>NIFEXQVDAQPLRPCELQRERAFLKREDYVPQCAEDGSFQTVQCGKDGASCWCVDADGREVPGSRQPGRPAACLSFCQLQKQQILLSSYINSTATSYLPQCQDSGDYSPVQCDLRRRQCWCVDAEGMEVYGTRQQGRPARCPRSCEIRNRRLLHGVGDRSPPQCSPDGAFRPVQCKFVNTTDMMIFDLVHSYSRFPDAFVTFSSFRSRFPEVSGYCYCADSQGRELAETGLELLLDEIYDTIFAGLDLASTFAETTLYRILQRRFLAVQLVISGRFRCPTKCEVERFAATSFRHPYVPSCHPDGEYQAAQCQQGGPCWCVDSRGQEIPGTRQRGEPPSCAEDQSCPSERRRAFSRLRFGPSGYFSRRSLLLAPEEGPVSQRFARFTASCPPSIKELFLDSGIFQPMLQGRDTRFVAPESLLKEAIRGLFPSRELARLALQFTTNAKRLQQNLFGGRFLVNVGQFNLSGALGTRGTFNFSHFFQQLGLPGFQDGRALADLAKPLSVGLNSNPASEAPKASKIDVALRKPVVGSFGFEVNLQENQNALQFLSSFLELPEFLLFLQHAISVPEDIARDLGDVMEMVFSSQGCGQAPGSLFVPACTAEGSYEEVQCFAGDCWCVDAQGRELAGSRVRGGRPRCPTECEKQRARMQSLLGSQPAGSSLFVPACTSKGNFLPVQCFNSECYCVDTEGQPIPGTRSALGEPKKCPSPCQLQAERAFLGTVRTLVSNPSTLPALSSIYIPQCSASGQWSPVQCDGPPEQAFEWYERWEAQNSAGQALTPAELLMKIMSYREAASRNFRLFIQNLYEAGQQGIFPGLARYSSFQDVPVSVLEGNQTQPGGNVFLEPYLFWQILNGQLDRYPGPYSDFSAPLAHFDLRSCWCVDEAGQKLEGTRNEPNKVPACPGSCEEVKLRVLQFIREAEEIVTYSNSSRFPLGESFLAAKGIRLTDEELAFPPLSPSRETFLEKFLSGSDYAIRLAAQSTFDFYQRRLVTLAESPRAPSPVWSSAYLPQCDAFGGWEPVQCHAATGHCWCVDGKGEYVPTSLTARSRQIPQCPTSCERLRASGLLSSWKQAGVQAEPSPKDLFIPTCLETGEFARLQASEAGTWCVDPASGEGVPPGTNSSAQCPSLCEVLQSGVPSRRTSPGYSPACRAEDGGFSPVQCDPAQGSCWCVLGSGEEVPGTRVAGSQPACESPQCPLPFSVADVAGGAILCERASGLGAAAGQRCQLRCSQGYRSAFPPEPLLCSVQRRRWESRPPQPRACQRPQFWQTLQTQAQFQLLLPLGKVCSADYSGLLLAFQVFLLDELTARGFCQIQVKTAGTPVSIPVCDDSSVKVECLSRERLGVNITWKLQLVDAPPASLPDLQDVEEALAGKYLAGRFADLIQSGTFQLHLDSKTFSADTSIRFLQGDRFGISPRTQFGCLEGFGRVVAASDASQDALGCVKCPEGSYFQDEQCIPCPAGFYQEQAGSLACVPCPEGRTTVYAGAFSQTHCVTDCQKNEVGLQCDQDGQYRASQRDRTSGKAFCVDGEGRRLPWTEAEAPLVDAQCLVMRKFEKLPESKVIFSADVAVMVRSEVPGSESSLMQCLADCALDEACGFLTVSTAGSEVSCDFYAWASDSIACTTSGRSEDALGTSQATSFGSLQCQVKVRSREGDPLAVYLKKGQEFTITGQKRFEQTGFQSALSGMYSPVTFSASGASLAEVHLFCLLACDHDSCCDGFILVQVQGGPLLCGLLSSPDVLLCHVRDWRDPAEAQANASCPGVTYDQDSRQVTLRLGGQEIRGLTPLEGTQDTLTSFQQVYLWKDSDMGSRSESMGCRRDTEPRPASPSETDLTTGLFSPVDLIQVIVDGNVSLPSQQHWLFKHLFSLQQANLWCLSRCAGEPSFCQLAEVTDSEPLYFTCTLYPEAQVCDDILESSPKGCRLILPRRPSALYRKKVVLQDRVKNFYNRLPFQKLTGISIRNKVPMSDKSISSGFFECERLCDMDPCCTGFGFLNVSQLKGGEVTCLTLNSLGLQTCSEEYGGVWRILDCGSPDTEVRTYPFGWYQKPVSPSDAPSFCPSVALPALTENVALDSWQSLALSSVIVDPSIRNFDVAHISTAAVGNFSAARDRCLWECSRHQDCLVTTLQTQPGAVRCMFYADTQSCTHSLQAQNCRLLLHEEATYIYRKPNIPLPGFGTSSPSVPIATHGQLLGRSQAIQVGTSWKPVDQFLGVPYAAPPLGEKRFRAPEHLNWTGSWEATKPRARCWQPGIRTPTPPGVSEDCLYLNVFVPQNMPPNASVLVFFHNAAEGKGSGDRPAVDGSFLAAVGNLIVVTASYRTGIFGFLSSGSSELSGNWGLLDQVVALTWVQTHIQAFGGDPRRVTLAADRGGADIASIHLVTTRAANSRLFRRAVLMGGSALSPAAVIRPERARQQAAALAKEVGCPSSSVQEMVSCLRQEPARILNDAQTKLLAVSGPFHYWGPVVDGQYLRETPARVLQRAPRVKVDLLIGSSQDDGLINRAKAVKQFEESQGRTSSKTAFYQALQNSLGGEAADAGVQAAATWYYSLEHDSDDXASFSRALEQATRDYFIICPVIDMASHWARTVRGNVFMYHAPESYSHSSLELLTDVLYAFGLPFYPAYEGQFTLEEKSLSLKIMQYFSNFIRSGNPNYPHEFSRRAPEFAAPWPDFVPRDGAESYKELSVLLPNRQGLKKADCSFWSKYIQSLKASADETKDGPSADSEEEDQPAGSGLTEDLLGLPELASKTYSK[2x]

Thyroglobulin (Tg) is a 660 kDa (2 × 330 kDa) homodimeric protein which is the most highly expressed protein in the thyroid gland. The protein is secreted by thyrocytes into the thyroid follicle lumen where, upon iodination by thyroid peroxidase, Tg functions as a scaffold protein for thyroid hormonogenesis and as a storage protein for both thyroid hormones and iodide. An oxidative coupling reaction in which a diiodotyrosine (DIT) acceptor receives (via a covalent quinol-ether linkage) the iodophenolic ring of a neighboring DIT donor results in the formation of thyroxine at an acceptor site and dehydroalanine at the corresponding donor site. Tg is a homodimeric protein packed with multiple Tg type 1 (Tg1) repeating structural motifs.

Here, a three-dimensional cryoEM reconstruction of bovine thyroglobulin at an overall resolution of 2.6 Å is presented. In this report, we present a high-resolution structure of purified Tg (iodinated in vivo with normal iodide content) from the bovine thyroid gland. We have been able to definitively identify three (of 70) tyrosine side chains per Tg monomer that are modified either to diiodotyrosine or thyroxine (Tyr24 and Tyr2575, indicative of acceptor sites). In addition, we observe four tyrosines with no discernible side chain despite well defined main-chain density, which we have tentatively assigned as dehydroalanines (Tyr89, Tyr149, Tyr1395 and Tyr2542); these are the only identifiable candidates as donors in thyroid hormone formation. Nevertheless, two acceptor–donor pairs were clearly identified in the structure, involving Tyr24 (acceptor)–Tyr149 (donor) and Tyr2542 (donor)–Tyr2575 (acceptor). Our high-resolution cryoEM map and model provide clear structural evidence for Tyr24–Tyr149 and Tyr2575–Tyr2542 functioning as acceptor–donor pairs. Both thyroxine acceptor sites at Tyr24 and Tyr2575 exhibited extra densities in the cryoEM map, revealing two phenolic rings coupled together, forming T4 at the site of the acceptor tyrosine. In contrast, Tyr149 exhibited no side-chain density in the cryoEM map, likely indicating the conversion of Tyr149 to dehydro­alanine. The distance between the Tyr24–Tyr149 acceptor–donor pair is 27.4 Å (Cα–Cα) in our structure in which thyroxine has already been formed. The second iodotyrosyl coupling site, where the donor Tyr2542 and the acceptor Tyr2575 are located, depicts a similar mechanism in reverse. When compared with the non-iodinated human Tg cryoEM structure, the α-helix with Tyr2542 has been slightly unwound and rotated, resulting in a 7 Å shift from its relative position in non-iodinated Tg, effectively creating the binding pocket for T4 at Tyr2575.1,2-DIOCTANOYL-SN-GLYCERO-3-PHOSPHOCHOLINE | C24 H49 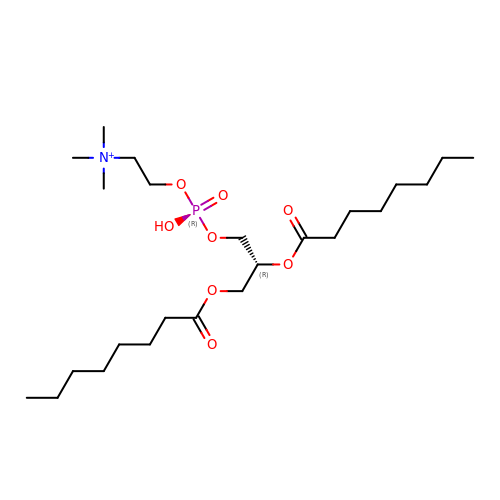N O8 P | YHIXRNNWDBPKPW-JOCHJYFZSA-O>[3x]MPMILGYWDIRGLAHAIRLLLEYTD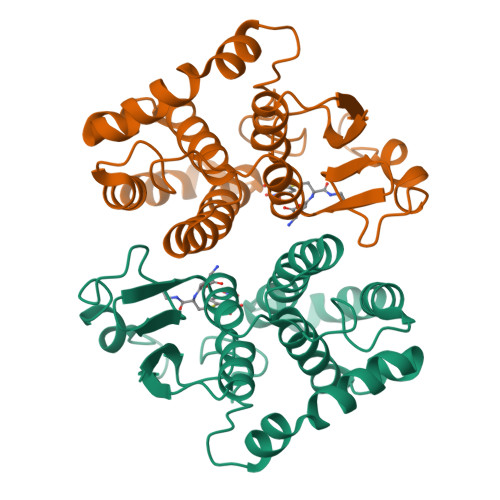SSYEEKKYTMGDAPDYDRSQWLNEKFKLGLDFPNLPYLIDGAHKITQSNAILCYIARKHNLCGETEEEKIRVDILENQTMDNHMQLGMICYNPEFEKLKPKYLEELPEKLKLYSEFLGKRPWFAGNKITFVDFLVYDVLDLHRIFEPKCLDAFPNLKDFISRFEGLEKISAYMKSSRFLPRPVFSKMAVWGNK>MDPYKEFGATVELLSFLPSDFFPSVRDLLDTASALYREALESP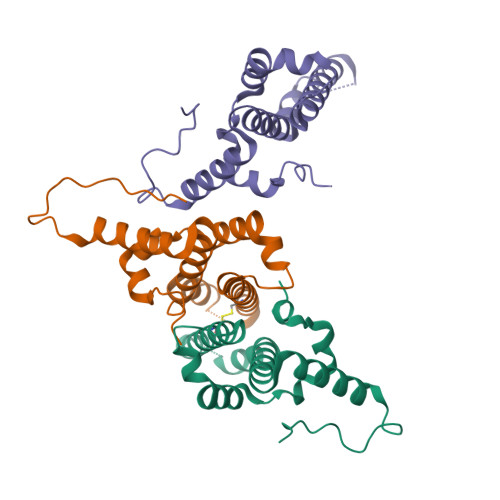EHCSPHHTALRQAILCWGELMTLATWVGGNLEDGSGTSGSSGSGSGGSGSGGGGELSLLTEVETPIRNEWGSRSNDSSDDLSLLTEVETPIRNEWGSRSNDSSDDLSLLTEVETPIRNEWGSRSNDSSDDLSLLTEVETPIRNEWGSRSNDSSDDIGTSGSSGSGSGGSGSGGGGGPSRDLVVSYVNTNMGLKFRQLLWFHISCLTFGRETVIEYLVSFGVWIRTPPAYRPPNAPILSTLPETTVVC[3x]> RCEEETPSLLWGLDPVFLAFAKLYIRDILDMKESRQVPGVFLYNGHPIKQVDVLGTVIGVRERDAFYSYGVDDSTGVINCICWKKLNTESVSAAPSAARELSLT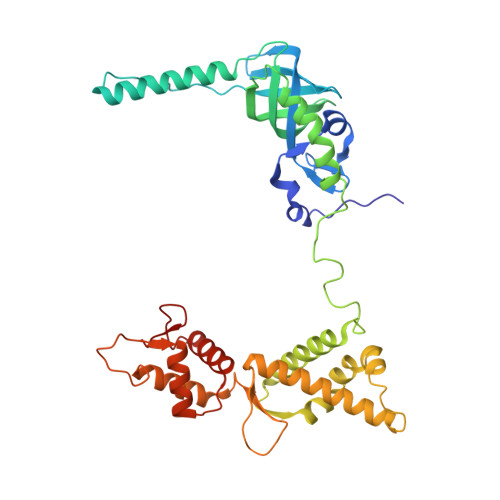SQLKKLQETIEQKTKIEIGDTIRVRGSIRTYREEREIHATTYYKVDDPVWNIQIARMLELPTIYRKVYDQPFHSSALEKEEALSNPGALDLPSLTSLLSEKAKEFLMENRVQSFYQQELEMVESLLSLANQPVIHSASSDQVNFKKDTTSKAIHSIFKNAIQLLQEKGLVFQKDDGFDNLYYVTREDKDLHRKIHRIIQQDCQKPNHMEKGCHFLHILACARLSIRPGLSEAVLQQVLELLEDQSDIVSTMEHYYTAF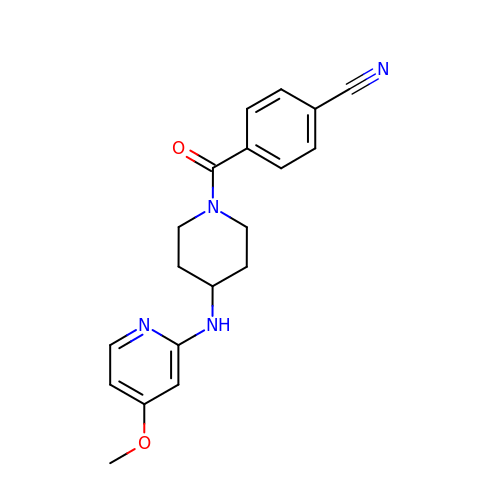4-({4-[(4-methoxypyridin-2-yl)amino]piperidin-1-yl}carbonyl)benzonitrile | C19 H20 N4 O2 | SZUVGMCKKLJAFX-UHFFFAOYSA-N The TonB-dependent transporter FhuE is integrated in the outer membrane of Gram-negative bacteria and has been reported to scavenge these fungally produced coprogens. FhuE belongs to the TonB-dependent transporter (TBDT) family and has been shown to be both necessary and sufficient for the utilization of fungally produced coprogens by Escherichia coli and other Gram-negative bacteria. Using this tool, it is shown that while FhuE is highly active in the import of coprogens, it has some level of promiscuity, acting as a low-affinity transporter for related siderophores. To determine the molecular basis for the transport of both high-affinity and low-affinity substrates by FhuE, we solved the crystal structure of FhuE in complex with Fe-coprogen. The structure of FhuE consists of a canonical TBDT fold consisting of a 22-stranded transmembrane β-barrel, the lumen of which is occluded by a globular plug domain [Fig. 3(a)].

Notably, all three hydroxamate groups of coprogen are coordinated by FhuE through two arginine residues (Arg117 and Arg142) and a tryptophan residue (Trp275). An additional hydrogen bond is observed between one of the keto O atoms of the coprogen diketopiperazine ring and an asparagine residue (Asn373), with the remainder of the binding pocket being composed of hydrophobic interactions [Fig. 3(b), Supplementary Fig. S5(b) and Supplementary Movie S1]. The planar nature of the FhuE binding pocket does not allow the coordination of the Fe-ferrichrome complex without significant clashes. The direct coordination via Arg142 of the hydroxamate groups appears to act as a selectivity filter, only allowing Fe-hydroxamate complexes in a planar configuration to be accommodated in the substrate-binding pocket [Figs. 3(b), 3(c) and 3(d)]. To determine the structural and biochemical basis for its selectivity and transport activity, we solved the crystal structure of FhuE in complex with coprogen. These data show that FhuE employs a selectivity filter in its substrate-binding site, making it specific for planar hydroxamate siderophores.

> APATEETVIVEGSATAPDDGENDYSVTSTSAGTKMQMTQRDIPQSVTIVSQQRMEDQQLQTLGEVMENTLGISKSQADSDRALYYSRGFQIDNYMVDGIPTYFESRWNLGDALSDMALFERVEVVRGATGLMTGTGNPSAAINMVRKHATSREFKGDVSAEYGSWNKERYVADLQSPLTEDGKIRARIVGGYQNNDSWLDRYNSEKTFFSGIVDADLGDLTTLSAGYEYQRIDVNSPTWGGLPRWNTDGSSNSYDRARSTAPDWAYNDKEINKVFMTLKQQFADTWQATLNATHSEVEFDSKMMYVDAYVNKADGMLVGPYSNYGPGFDYVGGTGWNSGKRKVDALDLFADGSYELFGRQHNLMFGGSYSKQNNRYFSSWANIFPDEIGSFYNFNGNFPQTDWSPQSLAQDDTTHMKSLYAATRVTLADPLHLILGARYTNWRVDTLTYSMEKNHTTPYAGLVFDINDNWSTYASYTSIFQPQNDRDSSGKYLAPITGNNYELGLKSDWMNSRLTTTLAIFRIEQDNVAQSTGTPIPGSNGETAYKAVDGTVSKGVEFELNGAITDNWQLTFGATRYIAEDNEGNAVNPNLPRTTVKMFTSYRLPVMPELTVGGGVNWQNRVYTDTVTPYGTFRAEQGSYALVDLFTRYQVTKNFSLQGNVNNLFDKTYDTNVEGSIVYGTPRNFSITGTYQF Recent findings revealed that TNIP1 functions as a checkpoint mechanism that fine-tunes the rate of mitophagy by disrupting the recycling of the ULK complex during autophagosome formation. The phosphorylation of the TNIP1 FIR motif enhances its binding affinity for FIP200, enabling TNIP1 to compete with other autophagy receptors, such as CCPG1 or Optineurin. Here, we determined several crystal structures of the FIP200 claw domain in complex with phosphorylated TNIP1 FIR peptides and elucidated the specific recognition of different phosphorylated TNIP1 by FIP200 claw domain. Each FIP200 claw domain within the dimer features a five-stranded antiparallel β-sheet and a short α-helix.

For the FIP200–TNIP1_pS123 complex, in an asymmetric unit, four FIP200 claw molecules assembled into two dimers, with each molecule binding to one TNIP1_pS123 peptide. The homodimerization of the FIP200 claw dimer primarily relies on the interaction between the N-terminal loop of one FIP200 claw domain and the corresponding loop of the other claw monomer. A portion of the TNIP1_pS123 peptide was observed, forming a short β-strand packing with β4 of the claw domain. Further structural analysis of the FIP200–TNIP1_pS123 complex revealed extensive polar interactions (charge–charge interactions and hydrogen bonding) and hydrophobic interactions. The FIP200 claw domain utilized its positively charged residues, R1573 and K1569 in the loop connecting β4 and β5, to specifically recognize the negatively charged N-terminal of TNIP1_pS123 peptide. Specifically, the ε-NH3+ group of K1569 side chain established specific charge–charge interactions to the phosphate group of TNIP1 pS123. R1573 formed specific charge–charge and hydrogen bonding interactions with the side chain of TNIP1 E104. Additionally, the side chains of F125 and V128, located within the conserved LC3 interaction region motif of TNIP1_pS123 peptide, inserted into two hydrophobic pockets of FIP200 claw domain. Moreover, the ε-NH3+ group of K1568 side chain formed a hydrogen bond with the carbonyl group of TNIP1 S122 main chain. As anticipated, the ITC results demonstrated that point mutations in crucial interface residues, including K1569A, R1573E, Y1564A, F1574A, and F1582A of FIP200, significantly abolished the specific interaction between the FIP200 claw domain and TNIP1_pS123 peptide.

>[4x]SRHSEKIAIRDFQVGDLVLIILDERHDNYVLFTVSPTLYFLHSESLPALDLKPGEGASGASRRPWVLGKVMEKEYCQAKKAQNRFKVPLGTKFYRVKAVSWNKKV;>SSGTSSEFEVV[4x]> GDPVEDIIHDALGSTARRAISSVTNAESAANTTPSSHRLETGRVPALQAAETGATSNATDENMIETRCVVNRNGVLETTINHFFSRSGLVGVVNLTDGGTDTTGYATWDIDIMGFVQLRRKCEMFTYMRFNAEFTFVTTTKNGEARPYMLQYMYVPPGAPKPTGRDAFQWQTATNPSVFVKLTDPPAQVSVPFMSPASAYQWFYDGYPTFGQHPETSNTTYGLCPNNMMGTFAVRVVSREASQLKLQTRVYMK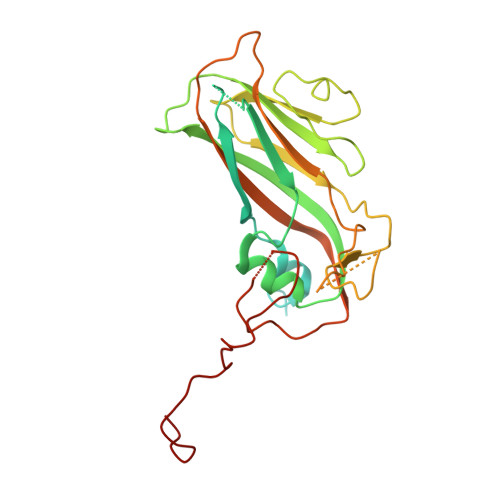LKHVRAWVPRPIRSQPYLLKNFPNYDSSKITNSARDRSSIKQANM> HPYYLRSFLVVLKTVLENEDDMLLFDEQEKGIVTKFYQLSATGQKLYVRLFQRKLSWIKMTKLEYEEIALDLTPVIEELTNAGFLQTESELQELSEVLELLSAPELKSLAKTFHLVNPNGQKQQLVDAFLKLAKQRSVCTWGKNKPGIGAVILKRAKALAGQSVRICKGPRAVFSRILLLFSLTDSMEDEDAACGGQGQLSTVLLVNLGRMEFPSYTINRKTHIFQDRDDLIRYAAATHMLSDISSAMANGNWEEAKELAQCAKRDWNRLKNHPSLRCHEDLPLFLRCFTVGWIYTRILSRFVEILQRLHMYEEAVRELESLLSQRIYCPDSRGRWWDRLALNLHQHLKRLEPTIKCITEGLADPEVRTGHRLSLYQRAVRLRESPSCKKFKHLFQQLPEMAVQDVKHVTITGRLCPQRGMCKSVFVMEAGEAADPTTVLCSVEELALAHYRRSGFDQGIHGEGSTFSTLYGLLLWDIIFMDGIPDVFRNACQAFPLDLCTDSFFTSRRPALEARLQLIHDAPEESLRAWVAATWHEQEGRVASLVSWDRFTSLQQAQDLVSCLGGPVLSGVCRHLAADFRHCRGGLPDLVVWNSQSRHFKLVEVKGPNDRLSHKQMIWLAELQKLGAEVEVCHVV;>MFEARLVQGSILKKVLEALKDLINEACWDISSSGVNLQSMDSSHVSLVQLTLRSEGFDTYRCDRNLAMGVNLTSMSKILKCAGNEDIITLRAEDNADTLALVFEAPNQEKVSDYEMKLMDLDVEQLGIPEQEYSCVVKMPSGEFARICRDLSHIGDAVVISCAKDGVKFSASGELGNGNIKLSQTSNVDKEEEAVTIEMNEPVQLTFALRYLNFFTKATPLSSTVTLSMSADVPLVVEYKIADMGHLKYYLAPKIE[3x]

FAN1 (FANCD2-FANCI-associated nuclease 1) is a DNA structure-dependent nuclease ubiquitously expressed in the central nervous system and peripheral tissues that plays a role in resolving interstrand crosslinks at replication forks. It possesses both 5′ flap endonuclease and 5′-3′ exonuclease activities, allowing it to process DNA structures that arise during replication stress and repair pathways. FAN1 comprises a DNA-binding SAF-A/B, Acinus and PIAS (SAP) domain, a tetratricopeptide repeat (TPR) domain that mediates dimerization and protein-protein interactions, a virus-type replication-repair nuclease module (VRR) containing the catalytic site, and an unstructured N-terminal region5. PCNA is a homotrimeric ring-shaped DNA clamp that encircles double-stranded DNA after being loaded by replication factor C (RFC).

To examine the role of PCNA on FAN1 activation, we solved the cryo-EM structures of a PCNA–FAN1–DNA complex. In contrast, this region remained unresolved in our previous structure of the FAN1–DNA complex, highlighting the critical role of PCNA in stabilizing FAN1. With this cryo-EM density map, we observed a direct interaction between R507 in FAN1 and D232 in PCNA. The salt bridge between R507 of FAN1 and D232 of PCNA stabilizes the FAN1-PCNA interface (left). Additional structural comparisons between the FAN1–DNA and FAN1–PCNA–DNA complexes revealed that the angle of the 5′ flap double-stranded DNA substrate remains fixed at 68°, and no significant conformational changes were observed in FAN1 between the two complexes. F Overall structural comparison between FAN1–PCNA–DNA (gray) and FAN1–DNA (black) complexes reveals no significant conformational changes in FAN1 upon binding to PCNA.> RERVKKEIKDLEKAKDFTEELIEKVKKYKALAREAALSKIGELASEIFAEFTEGKYSEVVVRAEEN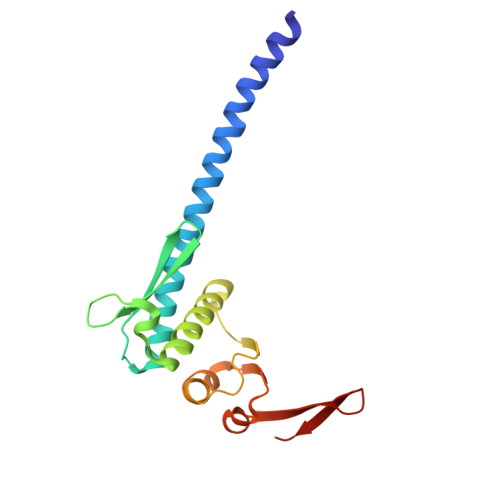KVRLFVVWEGKERPLTFLSGGERIALGLAFRLAMSLYLAGEISLLILDEPTPYLDEERRRKLITIMERYLKKIPQVILVSHDEELKDAADHVIRISLENGSSKVEVVS> MAKFEDKVDLYDDRGNLVEEQVPLEALSPLRNPAIKSIVQGIKRTVAVNLEGIENALKTAKVGGPACKIMGRELDLDIVGNAESIAAAAKEMIQVTEDDDTKVEL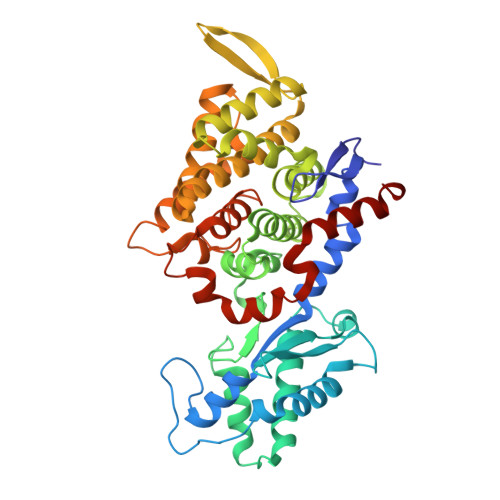LGGGKRALVQVPSARFDVAAEYSAAPLVTATAFVQAIINEFDVSMYDANMVKAAVLGRYPQSVEYMGANIATMLDIPQKLEGPGYALRNIMVNHVVATTLKNTLQAAALSTILEQTAMFEMGDAVGAFERMHLLGLAYQGMNADNLVFDLVKANGKEGTVGSVIADLVERALEDGVIKVEKELTDYKVYGTDDLAMWNAYAAAGLMAATMVNQGAARAAQGVSSTLLYYNDLIEFETGLPSVDFGKVEGTAVGFSFFSHSIYGGGGPGIFNGNHIVTRHSKGFAIPCVAAAMALDAGTQMFSPEATSGLIKEVFSQVDEFREPLKYVVEAAAEIKNEI> SMVKLANPLYTEWILEAIKKVKKQK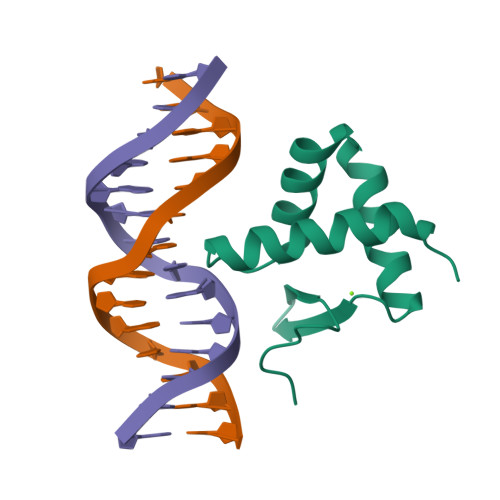QRPSEERICNAVSSSHGLDRKTVLEQLELSVKDGTILKVSNKGLNSYKDPDNPGRIALPKP> GPLGMATEEAIIRIPPYHYIHVLDQNSNVSRVEVGPKTYIRQDNERVLFAPVRMVTVPPRHYCIVANPVSRDAQSSVLFDVTGQVRLRHADQEIRLAQDPFPLYPGELLEKDITPLQVVLPNTALHLKALLDFEDKNGDKVMAGDEWLFEGPGTYIPQKEVEVVEIIQATVIKQNQALRLRARKECFDRDGKERVTGEEWLVRSVGAYLPAVFEEVLDLVDAVILTEKTALHLRARQNFKDLRGVAHRTGEEWLVTVQDTEAHVPDVYEEVLGVVPITTLGPRHYCVILDPMGPDGKNQLGQKRVVKGEKSFFLQPGERLERGIQDVYVLSEQQGLLLKALQPLEEGEGEERVA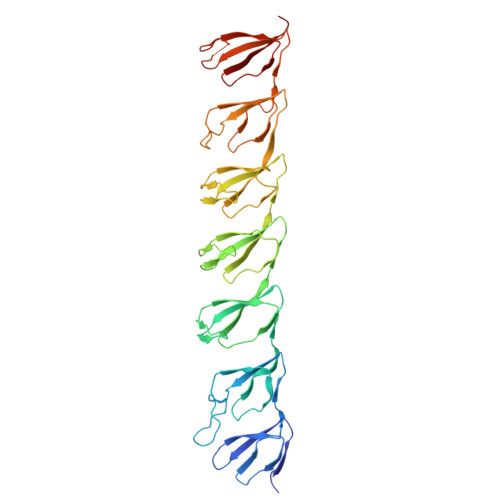HQAGDRWLIRGPLEYVPSAKVEVVEERQAIPLD>MAVAQDYLKVIWTAQEWSQDKVSTKMLAERIGVSASTASESIRKLAEQGLVDHEKYGAVTLTDSGRRAALAMVRRHRLLETFLVNELGYRWDEVHDEAEVLEHAVSDRLMARIDAKLGFPQRDPHGDPIPGADGQVPTPPARQLWACRDGDTGTVARISDADPQM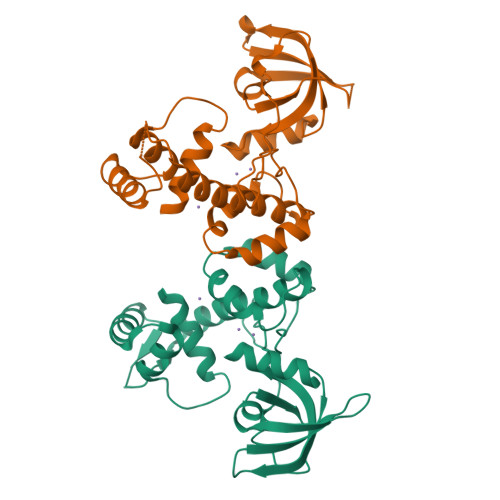LRYFASIGISLDSRLRVLARREFAGMISVAIDSADGATVDLGSPAAQAIWVVSLEHHHHHH[2x]3,5-BIS[(PHOSPHONOACETYL)AMINO]BENZOIC ACID | C11 H14 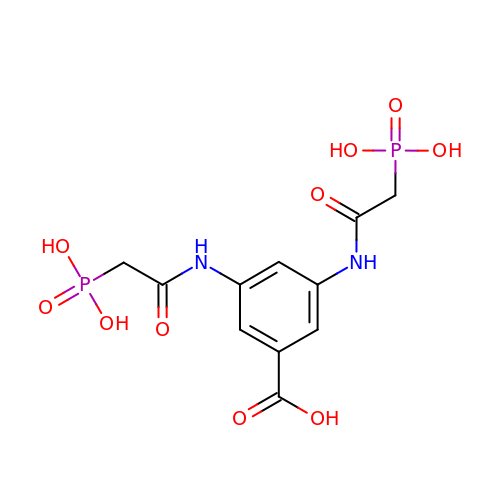N2 O10 P2 | LGLZCZRWQTWLGU-UHFFFAOYSA-N> MRAQRRFGLDLSWPRLTGVFLIDVAVLALVSHLPDAWQANHIAWWTGVGVAVLVTIVAVVTYRRTPLACALVARVLDRFVDPEMTLTEGCTPALDHQRRFGHDVVGIREYQGQLVAVVTVEGHEEAPSGRHRNRDAAPAWLPVEAVAARLRQFDVRLDAIDIVSVGTRRTSGRDDVSDVGVDDTGPVDARQPLDEHHTWLVLRMDPQRNVAAVAARDSVAATLAAATERLAHDLNGRRWTARPLTSSEIDDMDATVLAGLQPAHVRPRRRRLKYKQPEGYKEFVTSFWVSP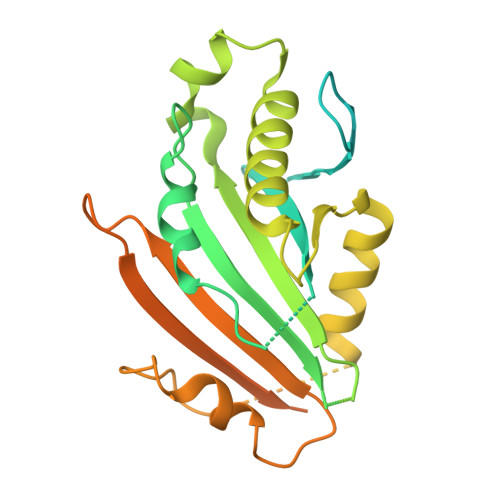RDITSETLERLWLPDTEATAVTVRLRPRHGGVEVSAWVRYHSSRRLRRSVWGGLNRLTGRQLDAVCASMPVPTRRPRLVVPARELHDGEELAVLVGQAPAPSPSPAAAR Non-ribosomal peptide synthetases are important enzymes for the assembly of complex peptide natural products. Within these multi-modular assembly lines, condensation domains perform the central function of chain assembly, typically by forming a peptide bond between two peptidyl carrier protein (PCP)-bound substrates. To address this, we report the structure and biochemical characterization of complexes of a PCP domain bearing a stable analog of the acyl acceptor complexed to the acceptor site of a C domain from the NRPS that biosynthesizes fuscachelin in the thermophile Thermobifida fusca. The C3 domain of the didomain resembles other members of its class, comprising a pseudo-dimer of CAT domains with bridge (R2923 to T2944) and floor loop (A2843 to L2858) regions.

To obtain crystals of the PCP2-C3 construct with this substrate analog (hereafter referred to as Glystab) bound, we again used Sfp to attach PPant-Glystab to the PCP domain. The overall structure of the Glystab-loaded PCP2-C3 construct was highly similar to the holo-PCP2C3 construct (572/532 Å2 buried surface area (chain A/B) excluding PPant). In the Glystab structure, however, the density for the PPant extends through the acceptor channel of the C domain into the active site, as observed in the structure of the R2577G mutant. R2577 now forms weak interactions with two of the carbonyl oxygen atoms in the PPant arm (3.7 Å and 3.8 Å), possibly acting as a ratchet to hold the PPant arm (and substrate) in the correct position until after peptide bond formation has occurred. The PPant-Glystab extends completely into the active site, with the terminal amine of Glystab stabilized by hydrogen-bond interactions. Of particular interest, given the lack of clarity over the role of the active site histidine in the HHxxxDE motif, is its close proximity (3.6 Å) to the amino group of the Glystab moiety. An ordered water molecule also sits close (2.9 Å) to this amino group, where it likely forms a hydrogen bond. We also observed the close interaction of the atypical E residue in the HHxxxDE motif (which is typically a Gly in most C-domains) with the nitrogen atom of Glystab (2.6 Å). It is important to note that Glystab sits in a different position to the aminoacyl mimic in a previous model of a C domain bound to the acceptor substrate – in these structures the aminoacyl mimic does not enter into the active site as far as observed in our GlyStab-PCP2-C3 complex. With a functional condensation assay in hand, we first could verify that the stabilized Glystab acceptor substrate was a functional mimic of Gly in this C domain using intact protein MS together with PPant ejection (see Methods section).

>VTAYEEIVCQVFAAVLDRSDVTADADFFALGGHSLLSLRVVARLRALLGVDVGVRDLFEAPTPAALAARLTTQTGRRPAVTRRGPDAPPVLSHFQRRLWLIEQVYQTRGAYNVPLAVHVSDRLDLDVLRAAVRDLVARHEVLRTLVRSSDDGPDPVLLAPEDAAVDVAEVQAAGPVADLLAELTAQPFDLATQIPLRVRMITGEQVDGCVLLLVCHHIAADEWSFAPLLRDLDTAYRARAAGRAPDWEPLPAQYSDYAATLHDWLGEATDPASPLRRQLDYWQHALQDLPDELDLPTDRPRPATASHRGGLARAELPPELVEAVRRLAAQHGVTVFMVVQAAVAVLLHRLGAGDDIPLGSPVADRADEAVHDTVGFFLNTLVLRVNLSGNPTFADLLDRVRAVDLEAFARADAPFDAVVDTVKPPRAVSRHPLFQTMVSYQRRPSDVDRLFGAATRLVEVPLDTAKFDLEFAFIEDGHGGAHIALNYAADLFDHDSAEQLVARLRTVLEHACADPCRPVAGVEVVSGA[2x]Talin (herein referring collectively to talin 1 and 2) couples the actomyosin cytoskeleton to integrins and transmits tension to the extracellular matrix. The N-terminal FERM domain of talin binds integrins, phosphatidylinositol 4,5-bisphosphate (PIP2), Arp2/3 and F-actin (at actin-binding site 1; ABS1), whereas the long C-terminal rod domain consisting of 13 α-helical bundles (R1–R13) contains two additional actin binding sites (ABS2 and ABS3; Atherton et al., 2015) and 11 vinculin-binding sites that are exposed upon force-mediated unfolding of the talin rod domains. Caskin2 is a relatively unexplored scaffold protein composed of six ankyrin repeats (ANK), an atypical Src homology 3 (SH3) domain and tandem sterile α-motifs (SAM) domains, followed by an extended disordered proline-rich region (PRR) and a conserved C-terminal domain (CTD). Here, we demonstrate that the scaffold protein Caskin2 interacts directly with the R8 domain of talin through its C-terminal LD motif.

Several proteins interact with talin via leucine-aspartic acid motifs (LD motifs) – short helical motifs that facilitate protein–protein interactions with the helical bundles of the talin rod domains – with the talin R7R8 domains being the best of the characterized talin LD-binding domains. Both Caskin1 and Caskin2 contain an LD motif in their conserved C-terminus, suggesting they might be binding partners of talin-R7R8. Using microscale thermophoresis (MST) we measured the affinity of the Caskin2-LD peptide to talin R7R8 as ∼2.7 µM. To further understand the mode of this interaction, we crystallized the complex and determined the crystallographic structure at 2.7 Å (1 Å=0.1 nm) resolution. The electron density map showed clear binding of the Caskin2-LD peptide to the R8 motif. The peptide was modeled, and the structure was refined to a Rfree of 26.9% with excellent geometry. The Caskin2-LD peptide was found to adopt a helical conformation that packs against two adjacent helices (α2 and α3) on the surface of the talin-R8 four-helix bundle, essentially forming a five-helix bundle. Analysis of the interaction interface showed that the buried interface area is 790 Å. The interaction is formed solely by van der Waals contacts between the talin-R8 and caskin2-LD helices, as hydrogen bonds are absent. The Caskin2 residues with the largest buried surface area are L1183 (120 Å), F1190 (113 Å), L1197 (105 Å) and L1201 (104 Å).

> GPGQKECDNALRQLETVRELLENPVQPINDMSYFGCLDSVMENSKVLGEAMTGISQNAKNGNLPEFGDAIATASKALCGFTEAAAQAAYLVGVSDPNSQAGQQGLVEPTQFARANQAIQMACQSLGEPGCTQAQVLSAATIVAKHTSALCNSCRLASARTANPTAKRQFVQSAKEVANSTANLVKTIKALDGDFTEENRAQCRAATAPLLEAVDNLSAFASNPEFSSVPAQISPEGRAAMEPIVISAKTMLESAGGLIQTARALAVNPRDPPRWSVLAGHSRTVSDSIKKLITSMRDKAPGQL;> STKHILDDISTMFDALADQLDAMLD2-(1H-indol-3-yl)-N-{[(2R,3R,4R,5R,6S)-3,4,5-trihydroxy-6-methylpiperidin-2-yl]methyl}acetamide 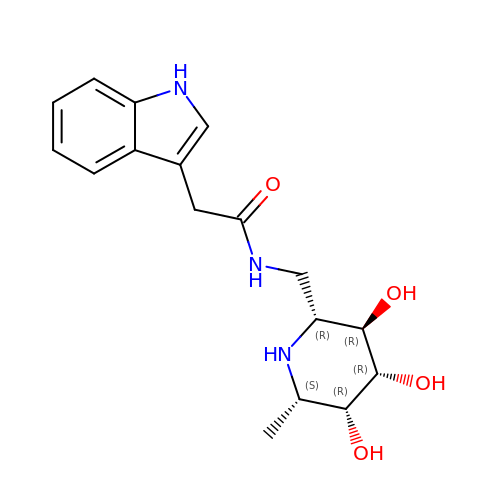| C17 H23 N3 O4 | SIWZFSDAFLUSGA-CXQPTDBTSA-N>SGSSMEGLAGYVYKAASEGKVLTLAALLLNRSESDIRYLLGYVSQQGGQRSTPLIIAARNGHAKVVRLLLEHYRVQTQQTGTVRFDGYVIDGATALWCAAGAGHFEVVKLLVSHGANVNHTTVTNSTPLRAACFDGRLDIVKYLVENNANISIANKYDNTCLMIAAYKGHTDVVRYLLEQRADPNAKAHCGATALHFAAEAGHIDIVKELIKWRAAIVVNGHGMTPLKVAAESCKADVVELLLSHADCDRRSRIEALELLGASFANDRENYDIMKTYHYLYLAMLERFQDGDNILEKEVLPPIHAYGNRTECRNPQELEAIRQDRDALHMEGLIVRERILGADNIDVSHPIIYRGAVYADNMEFEQCIKLWLHALHLRQKG[4x];>GRNKSSLLFKESEET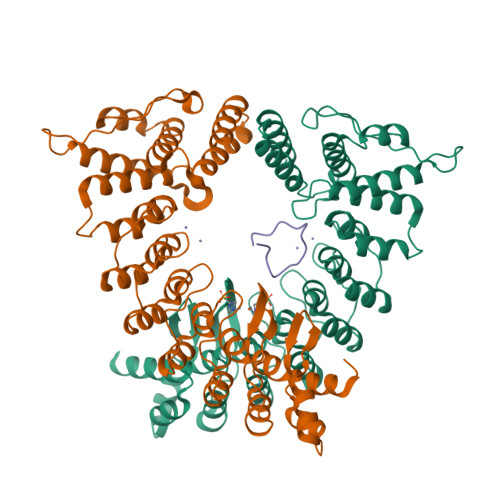RTPNCNCKYCSHPVLG[2x]> GPDGMAALSLPLPISAGRGYAPAFTLNYNSGAGNSPFGLGWDCNVMTIRRRTHFGVPHYDETDTFLGPEGEVLVVADQPRDESTLQGINLGATFTVTGYRSRLESHFSRLEYWQPKTTGKTDFWLIYSPDGQVHLLGKSPQARISNPSQTTQTAQWLLEASVSSRGEQIYYQYRAEDDTGCEADEITHHLQATAQRYLHIVYYGNRTASETLPG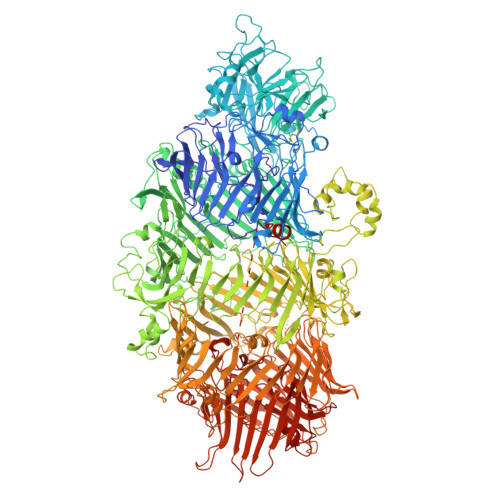LDGSAPSQADWLFYLVFDYGERSNNLKTPPAFSTTGSWLCRQDRFSRYEYGFEIRTRRLCRQVLMYHHLQALDSKITEHNGPTLVSRLILNYDESAIASTLVFVRRVGHEQDGNVVTLPPLELAYQDFSPRHHAHWQPMDVLANFNAIQRWQLVDLKGEGLPGLLYQDKGAWWYRSAQRLGEIGSDAVTWEKMQPLSVIPSLQSNASLVDINGDGQLDWVITGPGLRGYHSQRPDGSWTRFTPLNALPVEYTHPRAQLADLMGAGLSDLVLIGPKSVRLYANTRDGFAKGKDVVQSGDITLPVPGADPRKLVAFSDVLGSGQAHLVEVSATKVTCWPNLGRGRFGQPITLPGFSQPATEFNPAQVYLADLDGSGPTDLIYVHTNRLDIFLNKSGNGFAEPVTLRFPEGLRFDHTCQLQMADVQGLGVASLILSVPHMSPHHWRCDLTNMKPWLLNEMNNNMGVHHTLRYRSSSQFWLDEKAAALTTGQTPVCYLPFPIHTLWQTETEDEISGNKLVTTLRYARGAWDGREREFRGFGYVEQTDSHQLAQGNAPERTPPALTKNWYATGLPVIDNALSTEYWRDDQAFAGFSPRFTTWQDNKDVPLTPEDDNSRYWFNRALKGQLLRSELYGLDDSTNKHVPYTVTEFRSQVRRLQHTDSRYPVLWSSVVESRNYHYERIASDPQCSQNITLSSDRFGQPLKQLSVQYPRRQQPAINLYPDTLPDKLLANSYDDQQRQLRLTYQQSSWHHLTNNTVRVLGLPDSTRSDIFTYVAENVPAGGLNLELLSDKNSLIADDKPREYLGQQKTAYTDGQNTTPLQTPTRQALIAFTETTVFNQSTLSAFNGSIPSDKLSTTLEQAGYQQTNYLFPRTGEDKVWVAHHGYTDYGTAAQFWRPQKQSNTQLTGKITLIWDANYCVVVQTRDAAGLTTSAKYDWRFLTPVQLTDINDNQHLITLDALGRPITLRFWGTENGKMTGYSSPEKASFSPPSDVNAAIELKKPLPVAQCQVYAPESWMPVLSQKTFNRLAEQDWQKLYNARIITEDGRICTLAYRRWVQSQKAIPQLISLLNNGPRLPPHSLTLTTDRYDHDPEQQIRQQVVFSDGFGRLLQAAARHEAGMARQRNEDGSLIINVQHTENRWAVTGRTEYDNKGQPIRTYQPYFLNDWRYVSNDSARQEKEAYADTHVYDPIGREIKVITAKGWFRRTLFTPWFTVNEDENDTAAEVKKIDPKLYQKTPTVSVYDNRGLIIRNIDFHRTTANGDPDTRITRHQYDIHGHLNQSIDPRLYEAKQTNNTIKPNFLWQYDLTGNPLCTESIDAGRTVTLNDIEGRPLLTVTATGVIQTRQYETSSLPGRLLSVAEQTPEEKTSRITERLIWAGNTEAEKDHNLAGQCVRHYDTAGVTRLESLSLTGTVLSQSSQLLIDTQEANWTGDNETVWQNMLADDIYTTLSTFDATGALLTQTDAKGNIQRLAYDVAGQLNGSWLTLKGQTEQVIIKSLTYSAAGQKLREEHGNDVITEYSYEPETQRLIGIKTRRPSDTKVLQDLRYEYDPVGNVISIRNDAEATRFWHNQKVMPENTYTYDSLYQLISATGREMANIGQQSHQFPSPALPSDNNTYTNYTRTYTYDRGGNLTKIQHSSPATQNNYTTNITVSNRSNRAVLSTLTEDPAQVDALFDAGGHQNTLISGQNLNWNTRGELQQVTLVKRDKGANDDREWYRYSGDGRRMLKINEQQASNNAQTQRVTYLPNLELRLTQNSTATTEDLQVITVGEAGRAQVRVLHWESGKPEDIDNNQLRYSYDNLIGSSQLELDSEGQIISEEEYYPYGGTALWAARNQTEASYKTIRYSGKERDATGLYYYGYRYYQPWIGRWLSSDPAGTIDGLNLYRMVRNNPVTLLDPDGLNVFDEAILAALEP> MNGIHDT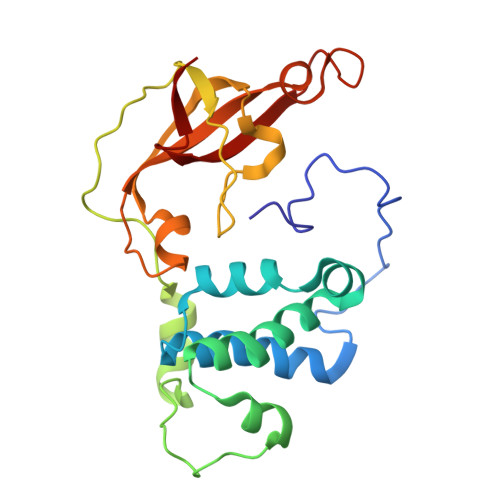GGAHGYGPVYREPNEPVFRYDWEKTVMSLLPALLANGNFNLDEFRHSIERMGPAHYLEGTYYEHWLHVFENLLVEKGVLTATEVATGKAASGKTATPVLTPAIVDGLLSTGASAAREEGARARFAVGDKVRVLNKNPVGHTRMPRYTRGKVGTVVIDHGVFVTPDTAAHGKGEHPQHVYTVSFTSVELWGQDASSPKDTIRVDLWDDFLEPA> GHMHDCHQVTVSRDVTLQNKERHDCNQVCASIDKETENKLNTDIIPRLTRYMSVKGNSIIAR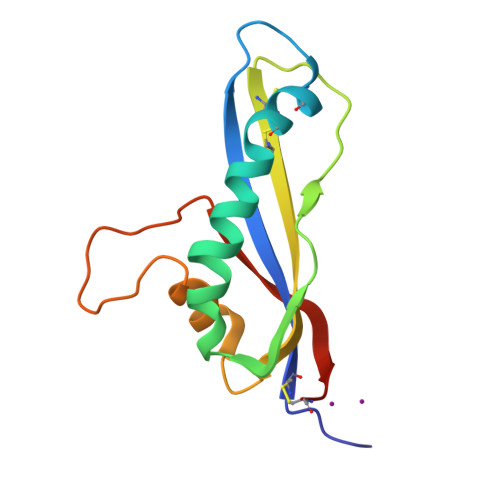VQQSNSDPKCSCTWRAIIWRVYKAYDENSLNVALHVSHPNQQIGENPDWSLVISNPNVHCLKH(2~{R},3~{R},4~{S},5~{R})-2-(6-aminopurin-9-yl)-5-ethyl-oxolane-3,4-diol 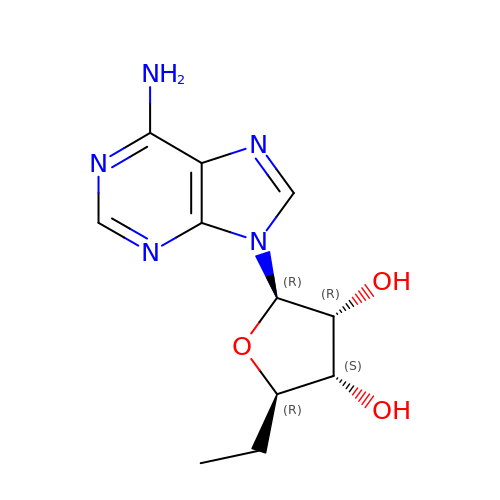| C11 H15 N5 O3 | RLOSCLOIJYLPHI-IOSLPCCCSA-N>[2x]AECSVDIQGNDQMQFNTNA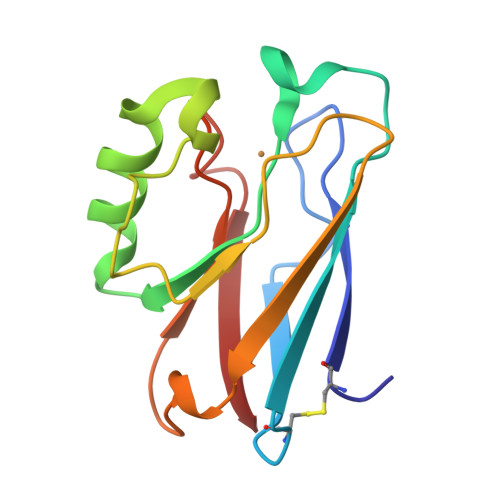ITVDKSCKQFTVNLSHPGNLPKNVMGHNWVLSTAADMQGVVTDGMASGLDKDYLKPDDSRVIAHTKLIGSGEKDSVTFDVSKLKEGEQYMFFCTPPGHSALMKGTLTLK> MSMDISDFYQT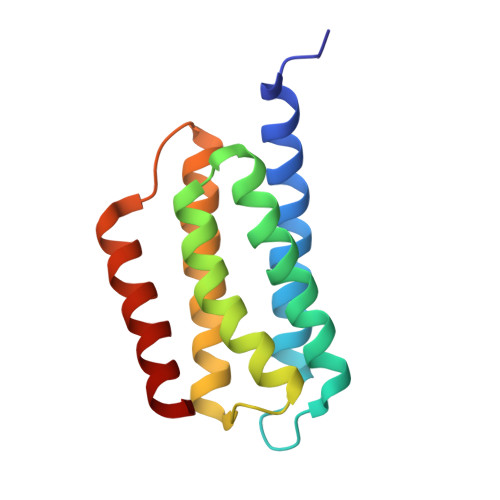FFDEADELLADMEQHLLVLQPEAPDAEQLNAIFRAAHSIKGGAGTFGFSVLQETTHLMENLLDEARRGEMQLNTDIINLFLETKDIMQEQLDAYKQSQEPDAASFDYICQALRQLALEAK> SPGMELQVSSGFVCNTCPEKWINFQRKCYYFGKGTKQWVHARYACDDMEGQLVSIHSPEEQDFLTKRASHTGSWIGLRNLDLKGEFIWVDGSHVDYSNWAPGEPTSRSQSEDCVMMRGSGRWNDAF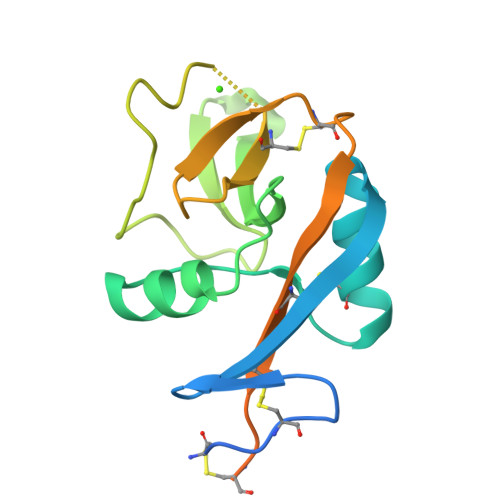CDRKLGAWVCDRLATCTPPASEGSAESMGPDSRPDPDGRLPTPSAPLHS>GRKERERLEEKLEDANERIAELVKLEERQRMARDLVDTLGQKLSLMGLKSDLARKLIYKDPEQAARELKSVQQTARTSLNEVRKIVSSMKGIRLKDELINIKQILEAADIMFIYEEEKWPENISL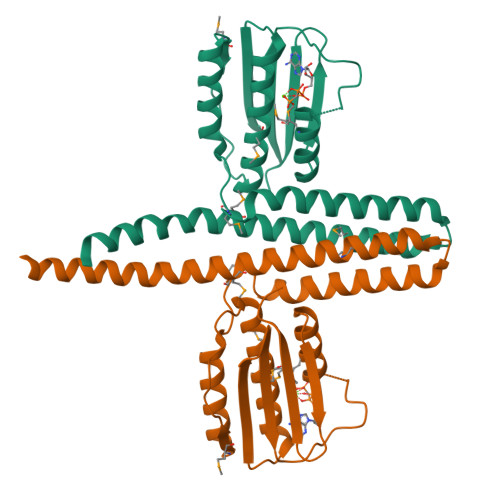LNENILSMCLKEAVTNVVKHSQAKTCRVDIQQLWKEVVITVSDDGTFKGEENSFSKGHGLLGMRERLEFANGSLHIDTENGTKLTMAIPNNSK[2x]> IPEYVDWRQKGAVTPVKNQGSCGSCWAFSAVVTIEGIIKIRTGNLNEYSEQELLDCDRRSYGCNGG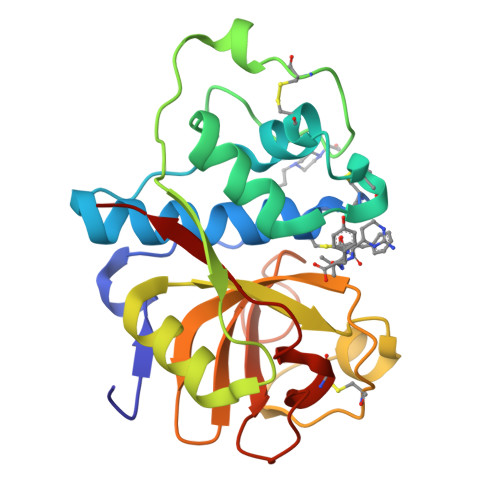YPWSALQLVAQYGIHYRNTYPYEGVQRYCRSREKGPYAAKTDGVRQVQPYNEGALLYSIANQPVSVVLEAAGKDFQLYRGGIFVGPCGNKVDHAVAAVGYGPNYILIKNSWGTGWGENGYIRIKRGTGNSYGVCGLYTSSFYPVKN> AEAGITGTWYNQLGSTFIVTAGADGALTGTYESAVGNAESRYVLTGRYDSA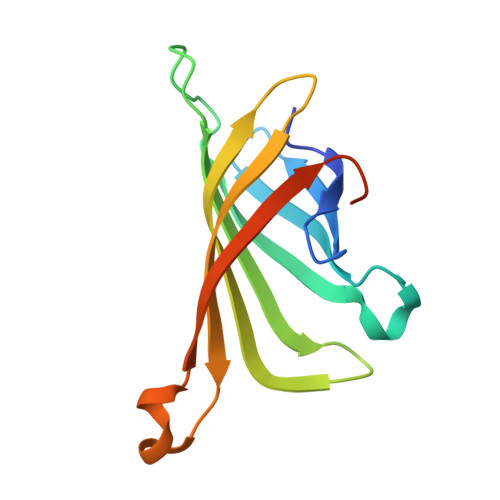PATDGSGTALGWTVAWKNNYRNAHSATTWSGQYVGGAEARINTQWLLTSGTTEANAWKSTLVGHDTFTKVKPSAASEEEEEE The protease-sensitive VP4 proteins protrude from the outer capsid shell, forming sixty spikes that are responsible for host receptor interactions. Each VP4 protein is cleaved by trypsin into two domains, VP5* and VP8*, corresponding to the stalk and the distal head of the spike protein, respectively. The distal VP8* head interacts with RV host glycan receptors for viral attachment, while the VP5* stalk assists in viral penetration into host cells. The RV VP8* domain adopts a classical galectin-like fold with the central structure being an anti-parallel β-sandwich formed by a five-stranded β-sheet and a six-stranded β-sheet.

The crystal structures of P (strain BM11596) and P (strain BM11596) in complex with LNFP I were solved. The VP8* of P BM11596 strain adopted a classical galectin-like fold as similar to other known VP8* structures, with two twisted antiparallel β-sheets consisting of strands A, L, C, D, G, H and M, B, I, J, K, respectively.

>[4x]VLDGPYQPTNFKPPNDYWILLNPTNQQVVLEGTNKTDIWVALLLVEPNVTNQSRQYTLFGETKQITVENNTNKWKFFEMFRSNVSAEFQHKRTLTSDTKLAGFMKFYNSVWTFHGETPHATTDYSSTSNLSEVETVIHVEFYIIPRSQESKCSEYINTG>[2x]HHHHHHSSGLVPRGSHMASMINIISRLQEVFGHAIKAAYPDLENPPLLVTPSQQAKFGDYQCNSAMGISQMLKTKEQKVNPREIAENITKHLPDNECIEKVEIAGPGFINVHLRKDFVSEQLTSLLVNGVQLPALGENKK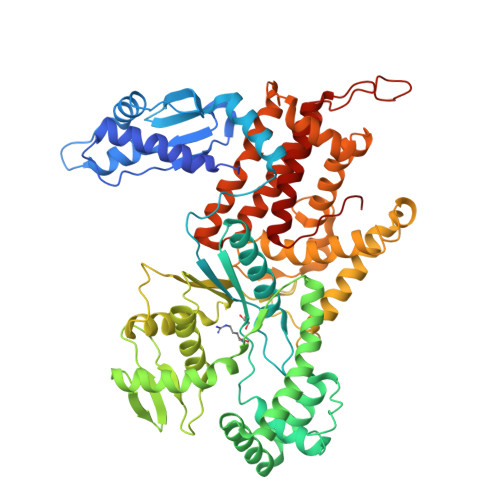VIVDFSSPNIAKEMHVGHLRSTIIGESISRLFEFAGYDVLRLNHVGDWGTQFGMLIAHLQDKFPDYLTVSPPIGDLQVFYKESKKRFDTEEEFKKRAYQCVVLLQGKNPDITKAWKLICDVSRQELNKIYDALDVSLIERGESFYQDRMNDIVKEFEDRGFVQVDDGRKIVFVPGCSIPLTIVKSDGGYTYDTSDLAAIKQRLFEEKADMIIYVVDNGQSVHFQTIFAAAQMIGWYDPKVTRVFHAGFGVVLGEDKKKFKTRSGETVRLMDLLGEGLKRSMDKLKEKERDKVLTAEELNAAQTSVAYGCIKYADLSRNRLNDYIFSFDKMLDDRGNTAAYLLYAFTRIRSIARLANIDEEMLQKAARETKILLDHEKEWKLGRCILRFPEILQKILDDLFLHTLCDYIYELATAFTEFYDSCYCVEKDRQTGKILKVNMWRMLLCEAVAAVMAKGFDILGIKPVQRM>MTEADVNPKAYPLADAHLTKKLLDLVQQSCNYKQLRKGANEATKTLNRGISEFIVMAADAEPLEIILHLPLLCEDKNVPYVFVR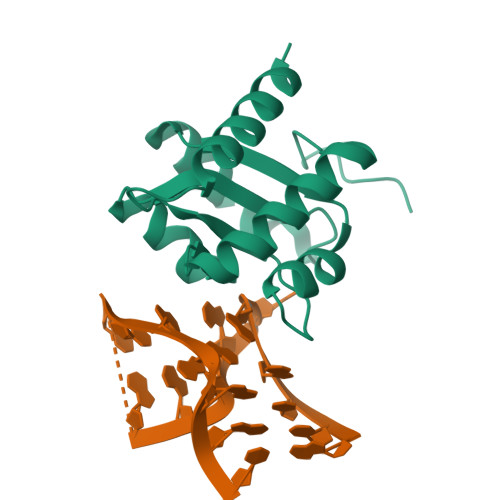SKQALGRACGVSRPVIACSVTIKEGSQLKQQIQSIQQSIERLLV[2x]> MKIDAIEAVIVDVPTKRPIQMSITTVHQQSYVIVRVYSEGLVGVGEGGSVGGPVWSAECAETIKIIVERYLAPHLLGTDAFNVSGALQTMARAVTGNASAK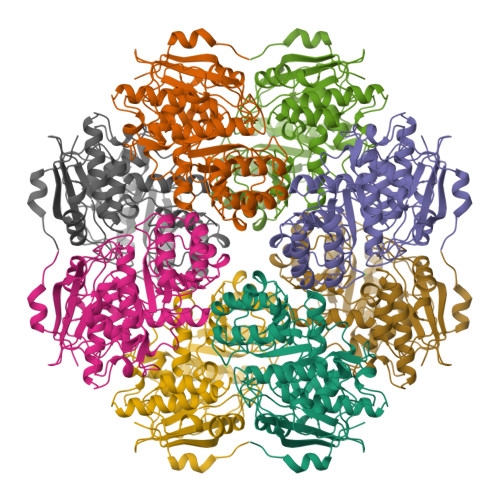AAVEMALLDLKARALGVSIAELLGGPLRSAIPIAWTLASGDTKRDLDSAVEMIERRRHNRFKVKLGFRSPQDDLIHMEALSNSLGSKAYLRVDVNQAWDEQVASVYIPELEALGVELIEQPVGRENTQALRRLSDNNRVAIMADESLSTLASAFDLARDRSVDVFSLKLCNMGGVSATQKIAAVAEASGIASYGGTMLDSTIGTSVALQLYSTVPSLPFGCELIGPFVLADTLSHEPLEIRDYELQVPTGVGHGMTLDEDKVRQYARVS4-[5-(4-tert-butylpiperazin-1-yl)pyridin-2-yl]-N-[(1R,2S,3S,5S,7s)-5-carbamoyltricyclo[3.3.1.1~3,7~]dec-2-yl]-3,4-dihydroquinoxaline-1(2H)-carboxamide 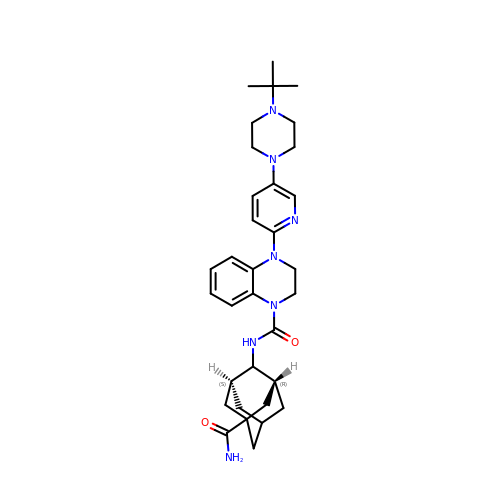| C33 H45 N7 O2 | RZUKTDWPBQOSBE-PKZLOJIYSA-N>[4x]MEMYFKRMKDEWTGLVEQADPPIRAKAAEIAVAHAHYLSIEFYRIVRIDPHAEEFLSNEQVERQLKSAMERWIINVLSAQVDDVERLIQIQHTVAEVHARIGIPVEIVEMGFRVL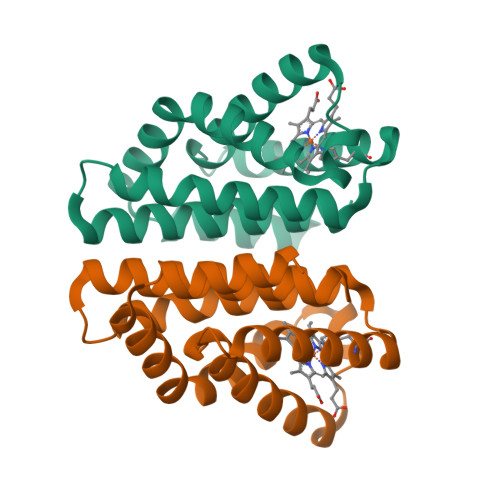KKILYPVIFSSDYSAAEKLQVYHFSINSIDIAMEVMTRAFLEHHHHHH>DAAQPALLQYHYDCGDFGMQLLAYPTRGRTVHFKVLDEFGTRFEVANCSICMHWLNTGEDGGLIFSAGYEGCHVLVKDGRYVLRVQLEEMLLSGVVAASYEVQMTCPRPAGYEILRDEKVHHHHHHHH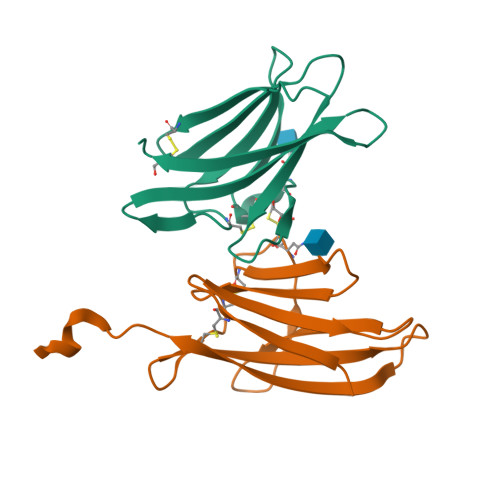QRPDRGNS[2x]> CTSIVAEDKKGHLIHGRNMDFGVFLGWNINNDTWVITEQLKPLTVNLDFQRNNKTVFKASSFAGYVGMLTGFKPGLFSLTLNERFSINGGYLGILEWILGKKDAMWIGFLTRTVLENSTSYEEAKNLLTKTKILAPAYFILGGNQSGEGCVITRDRKESLDVYELDAKQ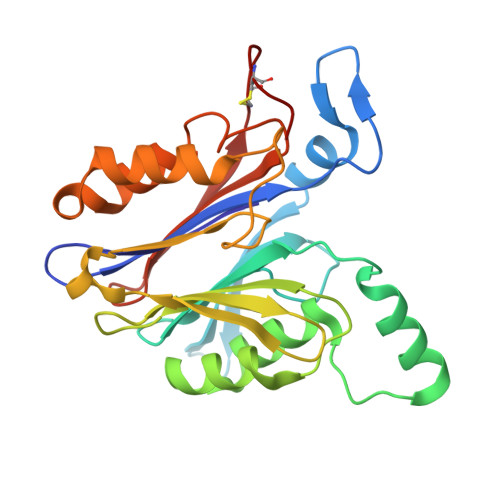GRWYVVQTNYDRWKHPFFLDDRRTPAKMCLNRTSQENISFETMYDVLSTKPVLNKLTVYTTLIDVTKGQFETYLRDCPDPCIGW>ARASPGSAASPRLREGPELSPDDPAGLLDLRQGMFAQLVAQNVLLIDGPLSWYSDPGLAGVSLTGGLSYKEDTKELVVAKAGVYYVFFQLELRRVVAGEGSGSVSLALHLQPLRSAAGAAALALTVDLPPASSEARNSAFGFQGRLLHLSAGQRLGVHLHTEARARHAWQLTQGATVLGLFRVTPEIPAGLPSPRSEHHHHHH[12x];>[12x]LQDPCSNCPAGTFCDNNRNQICSPCPPNSFSSAGGQRTCDICRQCKGVFRTRKECSSTSNAECDCTPGFHCLGAGCSMCEQDCKQGQELTKKGCKDCCFGTFNDQKRGICRPWTNCSLDGKSVLV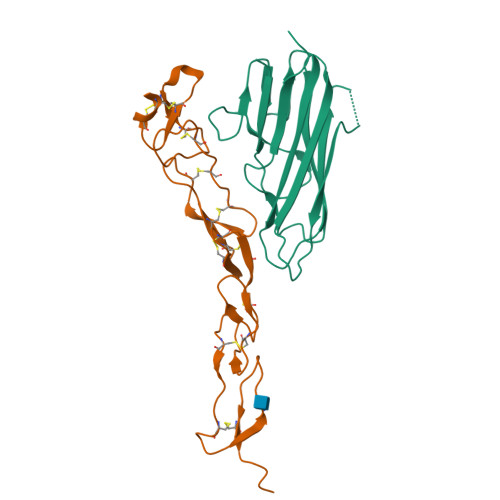NGTKERDVVCGPSPADLSPGASSVTPPAPAREHHHHHH>MFEIKKICCIGAGYVGGPTCSVIAHMCPEIRVTVVDVNESRINAWNSPTLPIYEPGLKEVVESCRGKNLFFSTNIDDAIKEADLVFISVNTPTKTYGMGKGRAADLKYIEACARRIVQNSNGYKIVTEKSTPVRAAESIRRIFDANTKPNLNLQVLSNPEFLAEGTAIKDLKNPDRVLIGGDETPEGQRAVQALCAVYEHWVPREKILTTNTWSSELSKLAANAFLAQRISSINSISALCEATGADVEEVATAIGMDQRIGNKFLKASVGFGGSCFQKDVLNLVYLCEALNLPEVARYWQQVIDMN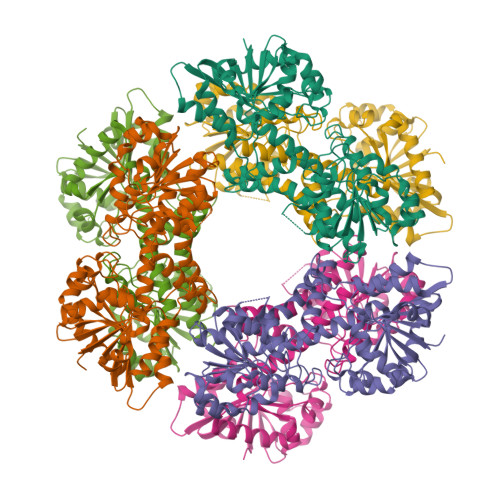DYQRRRFASRIIDSLFNTVTDKKIAILGFAFKKDTGDTRESSSIYISKYLMDEGAHLHIYDPKVPREQIVVDLSHPGVSEDDQVSRLVTISKDPYEACDGAHAVVICTEWDMFKELDYERIHKKMLKPAFIFDGRRVLDGLHNELQTIGFQIETIGKKVSSKRIPYAPSGEIPKFSLQDPPNKKPKV[3x]> MDLNATNYIRGCQSKTYDGKIFPGKGGEKQWICKDTIIHGDTNGACIPPRTQNLCVGELWDKSYGGRSNIKNDTKELLKEKIK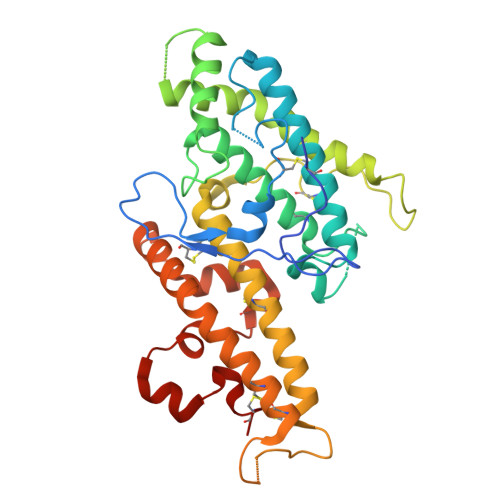NAIHKETELLYEYHDTGTAIISKNDKKGQKGKNDPNGLPKGFCHAVQRSFIDYKNMILGTSVNIYEHIGKLQEDIKKIIEKGTPQQKDKIGGVGSSTENVNAWWKGIEREMWDAVRCAITKINKKNNNSIFNGDECGVSPPTGNDEDQSVSWFKEWGEQFCIERLRYEQNIREACTINGKNEKKCINSKSGQGDKIQGACKRKCEKYKKYISEKKQEWDKQKTKYENKYVGKSASDLLKENYPECISANFDFIFNDNIEYKTYYPYGDYSSICSCEQVK>MANVNKTPGKTRRAEVAGGGFAGLTAAIALKQNGWDVRLHEKSSELRAFGAGIYLWHNGLRVLEGLGALDDVLQGSHTPPTYETWMHNKSVSKETFNGLPWRIMTRSHLHDALVNRARALGVDISVNSEAVAADPVGRLTLQTGEVLEADLIVGADGVGSKVRDSIGFKQDRWVSKDGLIRLIVPRMKKELGHGEWDNTIDMWNFWPRVQRILYSPCNENELYLGLMAPAADPRGSSVPIDLEVWVEMFPFLEPCLIEAAKLKTARYDKFETTKLDSW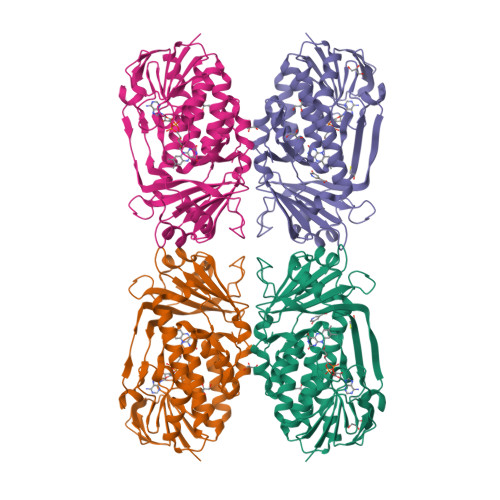TRGKVALVGDAAHAMCPALAQGAGCAMVNAFSLSQDLEEGSSVEDALVAWETRIRPITDRCQALSGDYAANRSLSKGNMFTPAALEAARYDPLRRVYSWPQ[2x]N-isobutyl-2-{[5-(thiophen-2-yl)-1,2-oxazol-3-yl]methoxy}acetamide 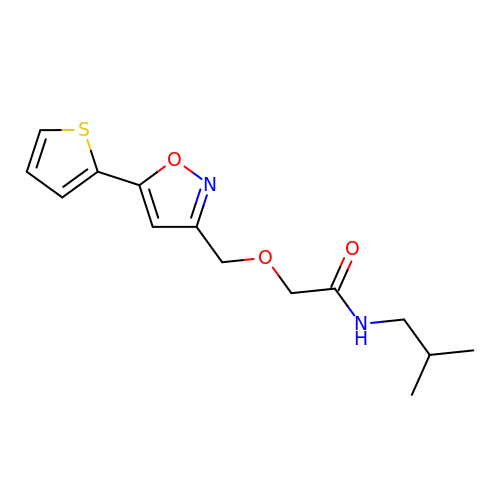| C14 H18 N2 O3 S | UJFGIBAYRIRNOV-UHFFFAOYSA-N> ATSDSNMLLNYVPVYVMLPLGVVNVDNVFEDPDGLKEQLLQL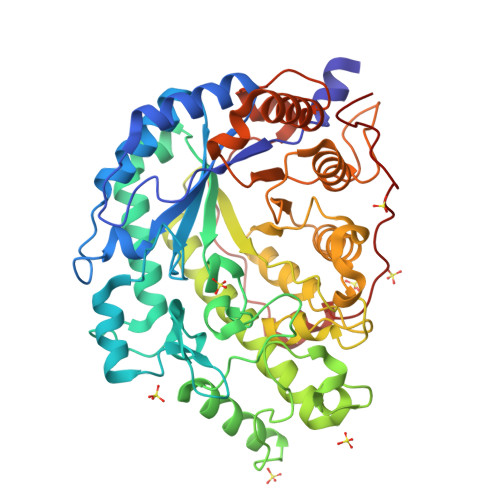RAAGVDGVMVDVWWGIIELKGPKQYDWRAYRSLLQLVQECGLTLQAIMSFHQCGGNVGDIVNIPIPQWVLDIGESNHDIFYTNRSGTRNKEYLTVGVDNEPIFHGRTAIEIYSDYMKSFRENMSDFLESGLIIDIEVGLGPAGELRYPSYPQSQGWEFPGIGEFQCYDKYLKADFKAAVARAGHPEWELPDDAGKYNDVPESTGFFKSNGTYVTEKGKFFLTWYSNKLLNHGDQILDEANKAFLGCKVKLAIKVSGIHWWYKVENHAAELTAGYYNLNDRDGYRPIARMLSRHHAILNFTCLEMRDSEQPSDAKSGPQELVQQVLSGGWREDIRVAGENALPRYDATAYNQIILNARPQGVNNNGPPKLSMFGVTYLRLSDDLLQKSNFNIFKKFVLKMHADQDYCANPQKYNHAITPLKPSAPKIPIEVLLEATKPTLPFPWLPETDMKVDG>[2x]GMSIEAKFKKLGTDNAPGQEVRQSAAGLEALIRGAP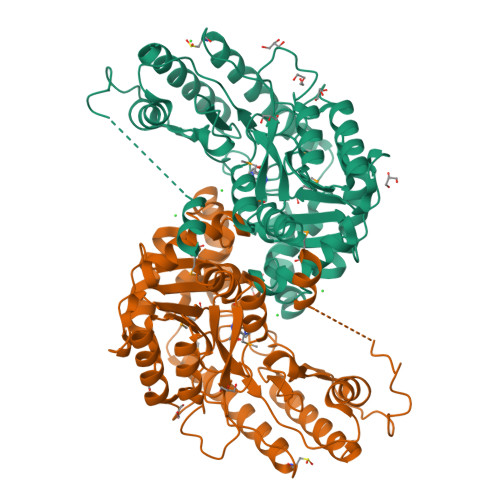IEGRPVDFSHGDVDAHEPTPGAFDLFSAGVQSGGVQAYTEYRGDLGIRDLLAPRLAAFTGAPVDARDGLIITPGTQGALFLAVAATVARGDKVAIVQPDYFANRKLVEFFEGEMVPVQLDYVSADETRAGLDLTGLEEAFKAGARVFLFSNPNNPAGVVYSAEEIGQIAALAARYGATVIADQLYSRLRYAGASYTHLRAEAAVDAENVVTIMGPSKTESLSGYRLGVAFGSRAIIARMEKLQAIVSLRAAGYSQAVLRGWFDEAPGWMEDRIARHQAIRDELLHVLRGCEGVFARTPQAGSYLFPRLPKLAVAPAEFVKILRLQAGVVVTPGTEFSPHTADSVRLNFSQDHEAAVAAARRIVTLVERYRA>[2x]GAMNAQAEEFKKYLETNGIKPKQFHKKELIFNQWDPQEYCIFLYDGITKLTSISENGTIMNLQYYKGAFVIMSGFIDTETSVGYYNLEVISEQATAYVIKINELKELLSKNLTH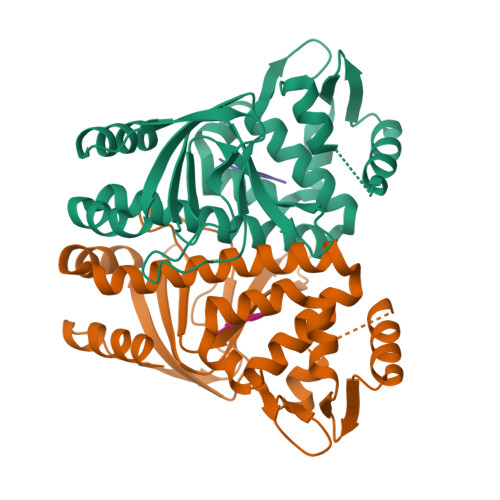FFYVFQTLQKQVSYSLAKFNDFSINGKLGSICGQLLILTYVYGKETPDGIKITLDNLTMQELGYSSGIAHSSAVSRIISKLKQEKVIVYKNSCFYVQNLDYLKRYAPKLDEWFYLACPATWGKLN;>[2x]EVFL The Ena/VASP proteins are a family of actin regulators involved in functions ranging from T-cell activation to axon guidance. There are three paralogs in mammals: ENAH (often called Mena), VASP, and EVL. All three proteins contain an N-terminal EVH1 interaction domain responsible for subcellular localization and a C-terminal EVH2 domain that polymerizes actin. The EVH1 domain binds SLiMs with the consensus motif [FWYL]PXΦP, where X is any amino acid and Φ is any hydrophobic residue.

To understand the structural basis for the high-affinity and selective interaction of PCARE B with ENAH, we solved a crystal structure of ENAH EVH1 domain fused to a 36-mer PCARE sequence to 1.65 Å resolution. To minimize the influence of the fusion on the domain–peptide interaction, we introduced a long, flexible linker between C-terminus of the ENAH EVH1 domain and the PCARE B sequence. Consistent with our truncation studies, our structure showed that only 21 residues of PCARE were fully resolved in the electron density (PCARE828–848). The high-resolution structure led to the surprising discovery that the LPPPP motif in PCARE binds at the expected canonical site, but in the opposite orientation from previously observed Ena/VASP EVH1 domains engaged with proline-rich peptides (Ball et al., 2000; Prehoda et al., 1999; Fedorov et al., 1999). PCARE828–848 uses a 14-residue alpha helix-rich extension C-terminal to the LPPPP motif to make additional contacts to an extended region on the EVH1 domain, explaining its high affinity. PCARE residues Phe843 and Leu846 make hydrophobic interactions with Ala83 and Pro65 on ENAH. The side chain of Asp840 on PCARE docks into a polar pocket on ENAH made up of the backbone atoms of ENAH residues Lys69 and Arg81. Most intriguing is the interaction between Val837 on PCARE and the hydrophobic groove in ENAH, which typically engages large aromatic residues. Interestingly, our structure of ENAH EVH1 domain bound to PCARE828–848 shows that 16 of the 18 residues that are within 4 Å of PCARE in ENAH are identical in ENAH ,VASP, and EVL. Specificity arises from a mechanism whereby PCARE stabilizes a conformation of the ENAH EVH1 domain that is inaccessible to family members VASP and EVL.

> SNAMSEQSICQARAAVMVYDDANKKWVPAGGSTGFSRVHIYHHTGNNTFRVVGRKIQDHQVVINCAIPKGLKYNQATQTFHQWRDARQVYGLNFGSKEDANVFASAMMHALEVLGGSGSGAAKSEELSCEMEGNLEHLPPPPMEVLMDKSFASLES8-OXOGUANINE 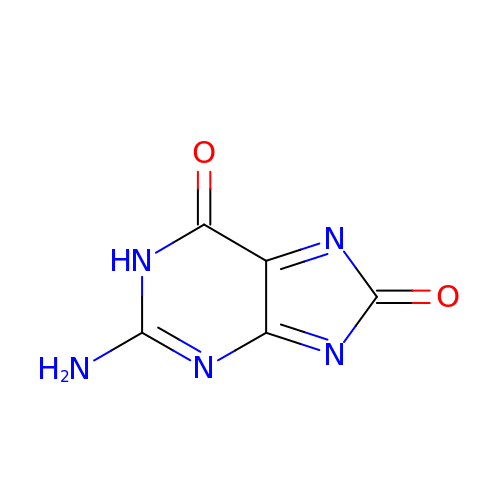| C5 H3 N5 O2 | UBKVUFQGVWHZIR-UHFFFAOYSA-N> GSELETDTREILEENNEMLHMYLNRLKTYQYLLKNEPIHVYYGSIDAYAEGIDKLLKTYADKMNLTASLCHYSTQADKDRLTEHMDDPADVQTRLDRKDVY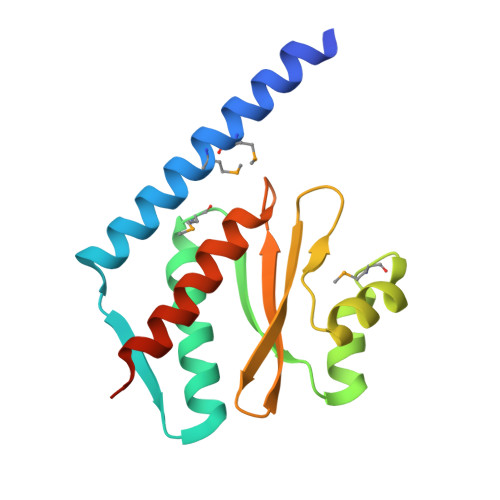YDQYGKVVLIPFTIETQNYVIKLTSDSIVTEFDYLLFTSLTSIYDLVLPIEEEGEG> EEYSSNWAGAVLIGDGYTKVTGEFTVPS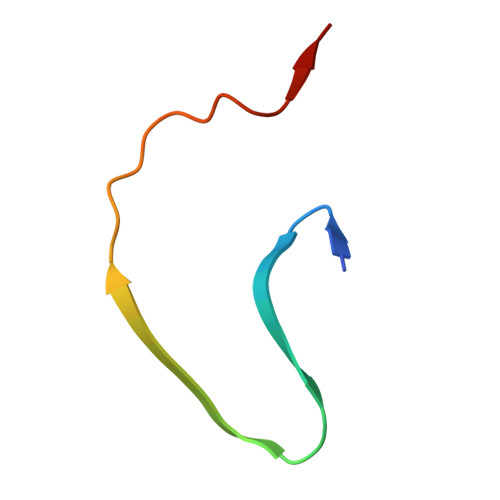VSAGSSGSSGY>[2x]MQVEQRTLNTAAHPFQITAYWLDQISDFETAVDYPIMIICPGGGFTYHSGREEAPIATRMMAAGMHTVVLNYQLIVGDQSVYPWALQQLGATIDWITTQASAHHVDCQRIILAGFSAGGHVVATYNGVATQPELRTRYHLDHYQGQHAAIILGYPVIDLTAGFPTTSAARNQITTDARLWAAQRLVTPASKPAFVWQ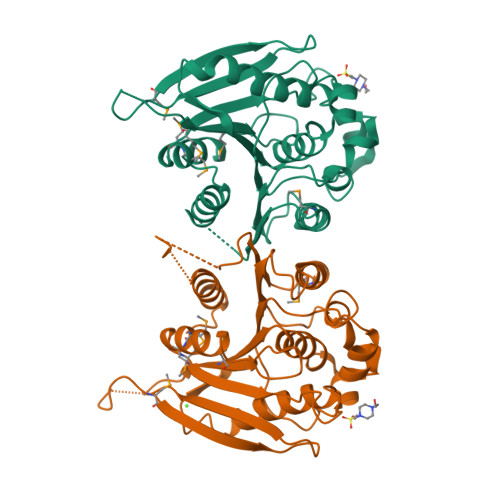TATDESVPPINSLKYVQAMLQHQVATAYHLFGSGIHGLALANHVTQKPGKDKYLNDQAAIWPQLALRWLQEQGLLAGNYLEHHHHHH>GSHMATPPKRSCPSFSASSEGTRIKKISIEGNIAAGKSTFVNILKQLCEDWEVVPEPVARWCNVQSTNVLQMMYEKPERWSFTFQTYACLSRIRAQLASLNGKLKDAEKPVLFFERSVYSDRYIFASNLYESECMNETEWTIYQDWHDWMNNQFGQSLELDGIIYLQATPET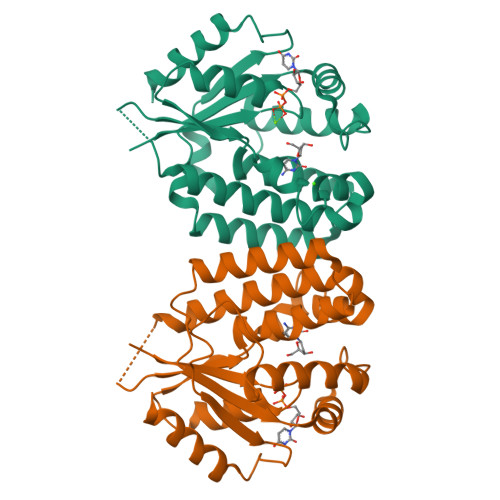CLHRIYLRGRNEEQGIPLEYLEKLHYKHESWLLHRTLKTNFDYLQEVPILTLDVNEDFKDKYESLVEKVKEFLSTL[4x]> SS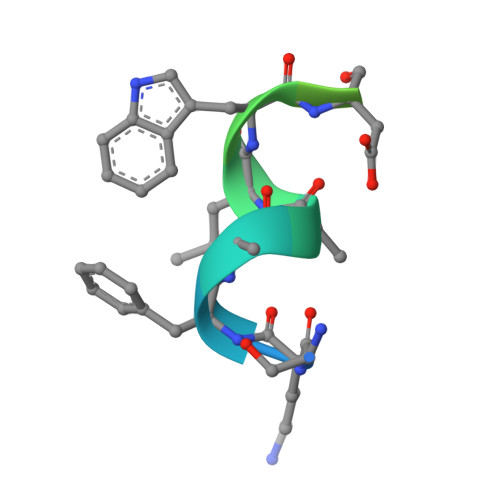KFAALWDPPKLSRSGSGK N-(6-{[1-(4-BROMOPHENYL)ISOQUINOLIN-6-YL]OXY}HEXYL)-N-METHYLPROP-2-EN-1-AMINE | C25 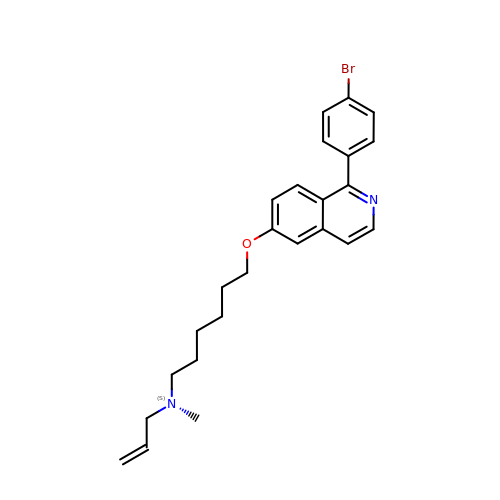H29 Br N2 O | PPLTVWUUFGVURW-UHFFFAOYSA-N>[2x]MDVLTKLLNRRFLPTIFKREIAHANRTGTPLSVLIIDVDKFKEINDTWGHNTGDEILRKVSQAFYDNVRSSDYVFRYGGDEFIIVLTEASENETLRTAERIRSR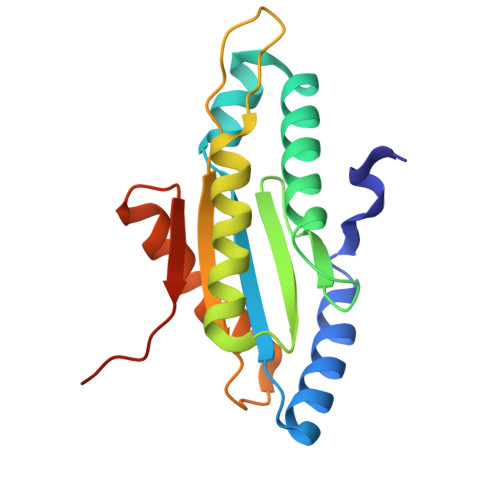VEKTKLKAANGEDIALSLSIGAAMFNGHPDYERLIQIADEALYIAKRRGRNRVELWKASLLEHHHHHH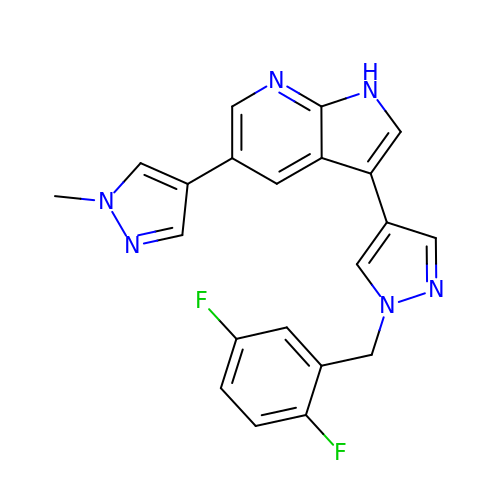3-[1-(2,5-difluorobenzyl)-1H-pyrazol-4-yl]-5-(1-methyl-1H-pyrazol-4-yl)-1H-pyrrolo[2,3-b]pyridine | C21 H16 F2 N6 | SDWMCZUOCJDBOJ-UHFFFAOYSA-N> GSHMTLKLYSFGPGANSLKPLATLYEKGLEFEQVFVDPSKFEQHSDWFKKINPRGQVPALWHDGKVVTESTVICEYLEDVFPESGNSLRPADPFKRAEMRVWTKWVDEYFCWCVSTIGWAFGIKAIAQKMSDEEFEEHINKNVPIPEQQLKWRRARNGFPQEMLDEEFRKVGVSVARLEETLSKQDYLVDTGYSLADICNFAIANGLQRP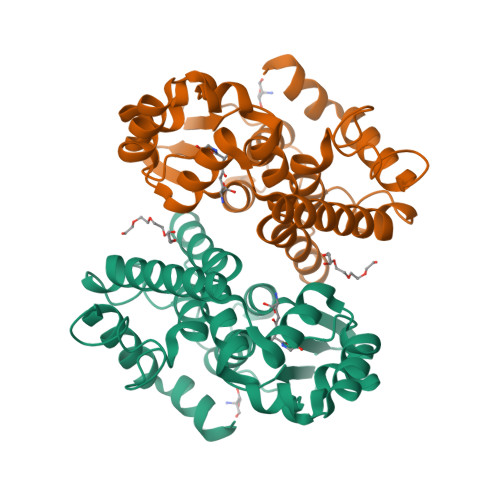GGFFGDYVNQEKTPGLCAWLDRINARPAIKEMFEKS>[2x]CGGGSFNNPSTIVIGQSKMIEKSDQSKDASAAKDDDNANADTKNKADSRLTMPVLGSVLAIPKRNQAYDKKKLTHLEEHVPLDENNITTAHTNPLPALTKELQERYEGGKIYQSDDKYKFVKAG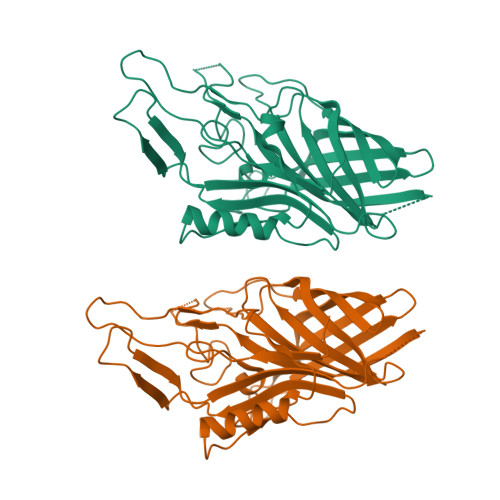WIFTGLRPDETIKTDEDTDQPKQYTKGDGYLYYYGDNPTTGLAKGVANYTGHWDFVTDVKRERESTITETTGRQAFGGGSGYKMDSGFGDEVGATSFAEQVFGQYAPRQGNHRAVFKADFDAKKLTGTLSTKQKAIASSPETYVDRYDIDATIKGNRFAGSAIAKNTKSSFLEPNFFNKNADNRLEGGFYGENAEELAGKFLTNDNSVFAVFAGKQD> GSARSSSYSGEYGSGGGKRFSHSGNQLDGPITALRVRVNTYYIVGLQVRYGKVWSDYVGGRNGDLEEIFLHPGES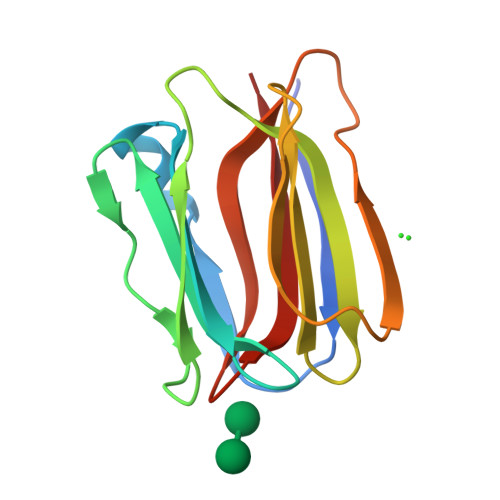VIQVSGKYKWYLKKLVFVTDKGRYLSFGKDSGTSFNAVPLHPNTVLRFISGRSGSLIDAIGLHWDV> GGRSGGRWIDGKHVPAPRNEKAEIAIFGVPEDPNFQSSGINFDNYDDIPVDASGKDVPEPITEFTSPPLDGLLLENIKLARFTKPTPVQKYSVPIVANGRDLMACAQTGSGKTGGFLFPVLSESFKTGPSPQPE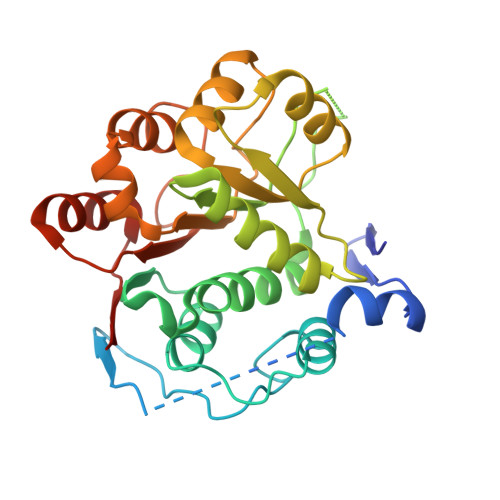SQGSFYQRKAYPTAVIMAPTRELATQIFDEAKKFTYRSWVKACVVYGGSPIGNQLREIERGCDLLVATPGRLNDLLERGKISLANVKYLVLDEADRMLDMGFEPQIRHIVEDCDMTPVGERQTLMFSATFPADIQHLARDFLSDYIFLSVGRVGS> MAVPFVEDWDLVQTLGEGAYGEVQLAVNRVTEEAVAVKIVDMKRAVDCPENIKKEICINKMLNHENVVKFYGHRREGNIQYLFLEYCSGGELFDRIEPDIGMPEPDAQRFFHQLMAGVVYLHGIGITHRDIKPENLLLDERDNLKISDFGLATVFRYNNRERLLNKMCGTLPYVAPELLKRREFHAEPVDVWSCGIVLTAMLAGELPWDQPSDSCQEYSDWKEKKTYLNPWKKIDSAPL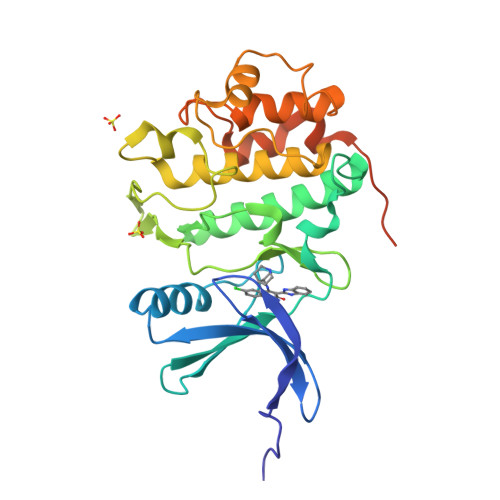ALLHKILVENPSARITIPDIKKDRWYNKPLKKGAKRPRVTSGGVSESPSGHHHHHH>MSQSVSERTRIKSDRYESGVIPYAKMGYWDAAYAVKNTDVLALFRITPQPGVDPVEAAAAVAGESSTATWTVVWTDLLTACDRYRAKAYRVDPVPNTTDQYFAFIAYECDLFEEGSLANLTASIIGNVFGFKAVSALRLEDMRIPHSYLKTFQGPATGVIVERERLNKYGIPLLGATVKPKLGLSGKNYGRVVYEGLKGGLDFLKDDENINSQPFMRWRERFLYCMEGINRASAATGETKGSYLNITAGTMEEVYKRAEYAKTVGSIVVMIDLVMGYTAIQSAAIWARDNDLILHLHRAGNSTYARQKNHGINFRVICKWMRMCGVDHIHAGTVVGKLEGDPLMIKGFYDTLLLTHLNVNLPYGIFFEMTWASLRKCMPVASGGIHCGQMHQLVHYLGDDVVLQFGGGTIGHPDGIQAGATANRVALEAMILARNEGADYFNSDIGPQILRNAAKTCGPLQTALDLWKDISFNYTSTDTSDFSVTPTANV[8x];>[8x]MRLTQGCFSFLPDLTDQQIEKQIAYCITKGWAMNVEWTDDPHPRNSYWELWGLPLFDVKDPASVMFELREARKSCAAGYIRINAFNAAYGTESCVMSFIVNRPSNEPGFYLERQELEGRRIAYTTKSYSVQANPEGGRY;>[8x]AAEWGSMNQ;>[4x]KWSPRGGS

pmcAlmost all biological CO2 fixation is catalyzed by ribulose 1,5-bisphosphate carboxylase/oxygenase (Rubisco), and about half of this activity is performed by marine photoautotrophs. To achieve significant local elevation of CO2 gas concentrations, the volume occupied by Rubisco needs to be minimized, which has led to the convergent evolution of the pyrenoid, a micron-sized, membraneless organelle of the chloroplast stroma. We report the identification and characterization of a diatom Rubisco-binding protein pyrenoid component 1 (PYCO1), which contains prion-like domains (PLD). The identification and characterization of PYCO1 indicates that the convergently evolved red pyrenoid matrix, like its counterpart in green algae, is formed by LLPS mediated by an intrinsically disordered repeat protein that contains multiple sticker motifs that bind to the Rubisco large and small subunits.

We determined the structure of the Rubisco–PYCO1(452 to 592) complex using cryo–electron microscopy. The resulting density map revealed that distinct PYCO1 motifs bind to both the small (Fig. 5D in blue; 2.6 Å resolution) and the large subunits (Fig. 5 E and F in magenta; 2.5 Å resolution) of Rubisco (2.0 Å resolution). Four instances of the previously identified sticker motif “KWSPRGGS” could be modeled into the density map surrounding Rubisco’s central solvent channel formed by the small subunits. The motifs adopt a helical conformation and collectively form a square-shaped plug of the central solvent channel. The indole group of each W476 binds to a groove formed by the “GGS” of the adjacent sticker, connecting the corners of the square. The interaction between the small subunits of Rubisco and the PYCO1 sticker tetrad is mediated by a network of hydrogen bonds. The structure revealed an additional interaction of the Rubisco large subunit with the PYCO1 fragment, the motif “AAEWGSMNQ” found near the C-terminus of PYCO1 (residues 577 to 585). The element adopted a helical conformation and bound to a largely hydrophobic cleft formed between the two domains of the large subunit near Rubisco’s dimer–dimer interface. The indole group of PYCO1 W580 is inserted into a hydrophobic pocket formed by LSU residues F102, F104, L361, F366, and F482. However, the interaction between Rubisco and these motifs is relatively weak because mutating the SSU-binding motif of PYCO1(452 to 592) was sufficient to eliminate the observed native PAGE shift.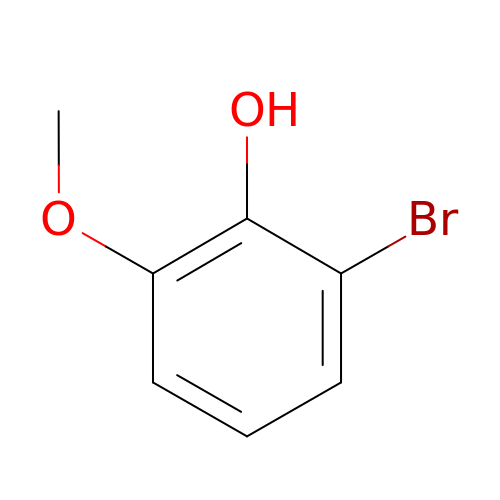2-bromo-6-methoxyphenol | C7 H7 Br O2 | WEUFQISIJPSTBM-UHFFFAOYSA-N>MEFRSLGRSGLSVSEIVYGNLLYPQDDTPDEVVLSSIRAALDAGVTTFDTADVYGMFRS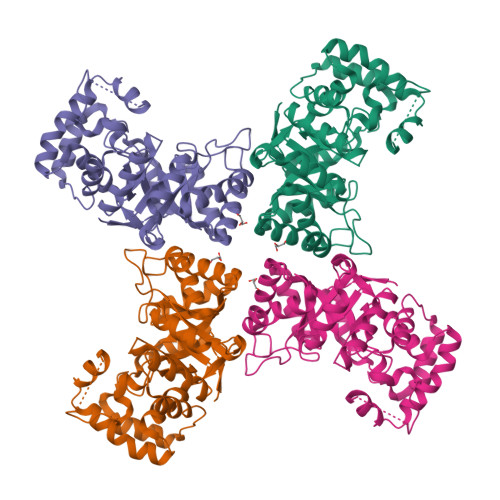ESLLGRALAGTPREELVLCTKVGMPTGFGPNGRGLSRKHVMESVDGSLRRLRVDHIDVYTAHRYDPATPLEELMWTFSDLVRAGKILYVGMSEWPVERIAEAAGIGARLGVPVICHMPRYSMLWRAPEAEVIPACRDLGIGQICYFTLEQGVLTGKYAPGAPPPAGSRATAPKGGRAPLMRRWLDDDKVLGRVERLRPLAEEAGLTTAQLALAWVLQNPGVSGAVIGSFNAEQVLANAESAGVRLETDLLVRIDEVLGDSVVHDEELEHHHHHH[2x]> SNAMTALKPALPDYLGNIRIILTRT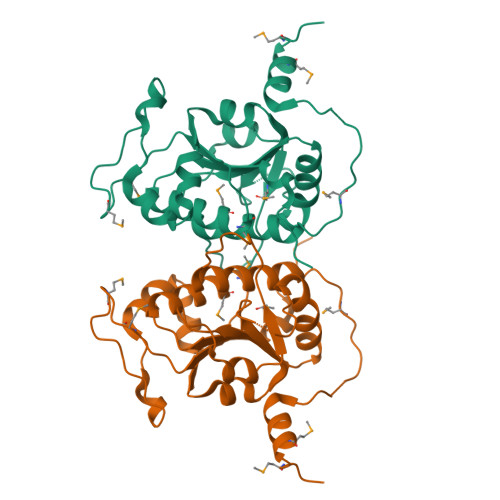SHPANIGSAARAMKTMGLHRLTIVTPNLMATPMTENPPVFNPDDVQSFALPEESFILASGAADVLHNAEIVATLDEALADTTIACALTSRRREITAPLQTPRDLVPELLQAANRGEKVALVFGNETFGLSIEEVRACNRLMTINGNPDYFSLNLAQAVQVVCYEIFSQTDSPMTHLQQEDHAATHEQIKGMLAHMESV>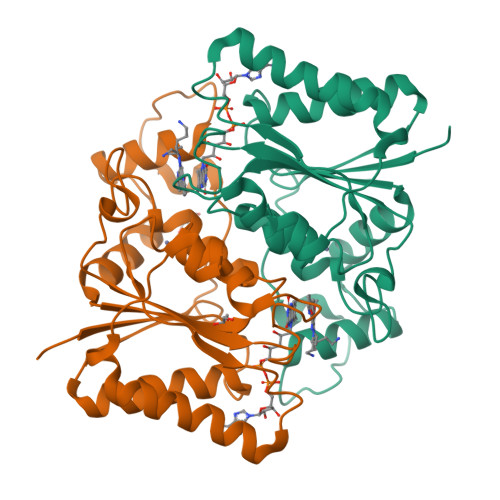[2x]GAMAGKKVLIVYAHQEPKSFNGSLKNVAVDELSRQGCTVTVSDLYAMNFEPRATDKDITGTLSNPEVFNYGVETHEAYKQRSLASDITDEQKKVREADLVIFQFPLYWFSVPAILKGWMDRVLCQGFAFDIPGFYDSGLLQGKLALLSVTTGGTAEMYTKTGVNGDSRYFLWPLQHGTLHFCGFKVLAPQISFAPEIASEEERKGMVAAWSQRLQTIWKEEPIPCTAHWHFGQ>[2x]DIVPMLETLKAFFDFGKDIKDDNYSNKLLDILSYLRNNQLYPGE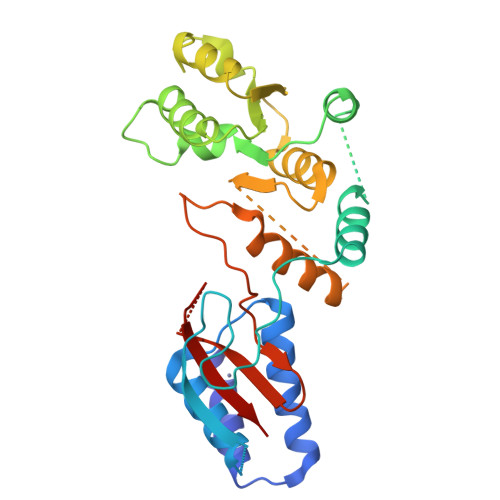SFAHSIKTWFESVPGKQWKGQFTTVRKSGQCSGCGKTIESIQLSPEEYECLKGKIMRDVIDGGDQYRKTTPQELKRFENFIKSRPPFDVVIDGLNVAKMFPKVRESQLLLNVVSQLAKRNLRLLVLGRKHMLRRSSQWSRDEMEEVQKQASCFFADDISEDDPFLLYATLHSGNHCRFITRDLMRDHKACLPDAKTQRLFFKWQQGHQLAIVNRFPGSKLTFQRILSYDTVVQTTGDSWHIPYDEDLVERCSCEVPTKWLCLHQKT(2S)-1-phenylpropan-2-amine | C9 H13 N | 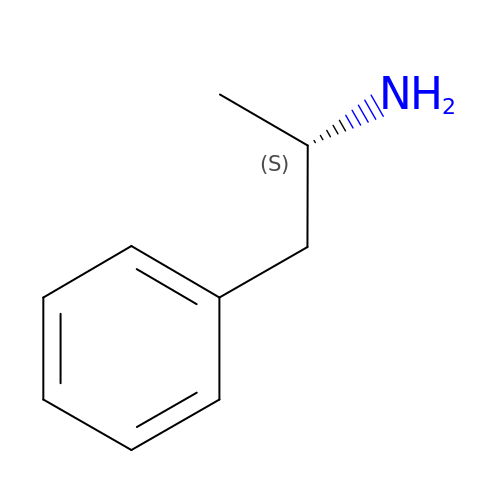KWTSXDURSIMDCE-QMMMGPOBSA-N> HHHHHHPEIVDTCSLASPASVCRTKHLHLRCSVDFTRRTLTGTAALTVQSQEDNLRSLVLDTKDLTIEKVVINGQEVKYALGERQSYKGSPMEISLPIALSKNQEIVIEISFETSPKSSALQWLTPEQTSGKEHPYLFSQCQAIHCRAILPCQDTPSVKLTYTAEVSVPKELVALMSAIRDGETPDPEDPSRKIYKFIQKVPIPCYLIALVVGALESRQIGPRTLVWSEKEQVEKSAYEFSETESMLKIAEDLGGPYVWGQYDLLVLPPSFPYGGMENPCLTFVTPTLLAGDKSLSNVIAHQISHSWTGNLVTNKTWDHFWLNEGHTVYLERHICGRLFGEKFRHFNALGGWGELQNSVKTFGETHPFTKLVVDLTDIDPDVAYSSVPYEKGFALLFYLEQLLGGPEIFLGFLKAYVEKFSYKSITTDDWKDFLYSYFKDKVDVLNQVDWNAWLYSPGLPPIKPNYDMTLTNACIALSQRWITAKEDDLNSFNATDLKDLSSHQLNEFLAQTLQRAPLPLGHIKRMQEVYNFNAINNSEIRFR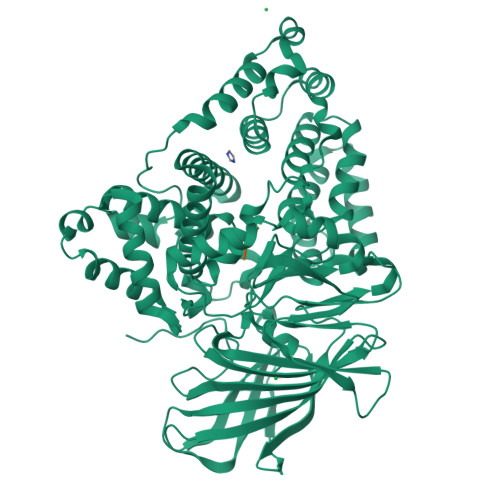WLRLCIQSKWEDAIPLALKMATEQGRMKFTRPLFKDLAAFDKSHDQAVRTYQEHKASMHPVTAMLVGKDLKVD;> RAR> F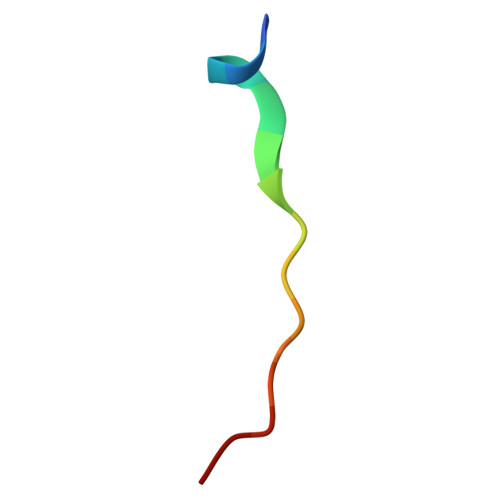RENVNAIRPFGRRP> RFILEISGDLACFTRSELKVERVSYPVITPAAARNILMAILWKPAIRWKVLKIEILKPIQWTNIRRNEVGTKMSERSG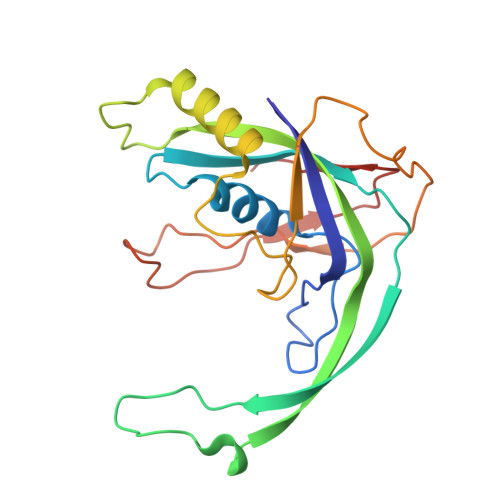SLYIEDNRQQRASMLLKDVAYRIHADFDMTSEAGESDNYVKFAEMFKRRAKKGQYFHQPYLGCREFPCDFRLLEKAEDGLPLEDITQDFGFMLYDMDFSKSDPRDSNNAEPMFYQCKAVNGVITVPP>GGEPAWDSPLRRVLAELNRIPSSRRRAARLFEWLIAPMPPDHFYRRLWEREAVLVRRQDHTYYQGLFSTADLDSMLRNEEVQFGQHLDAARYINGRRETLNPPGRALPAAAWSLYQAGCSLRLLCPQAFSTTVWQFLAVLQEQFGSMAGSNVYLTPPNSQGFAPHYDDIEAFVLQLEGRKLWRVYRPRVPTEELALTSSPNFSQDDLGEPVLQTVLEPGDLLYFPRGFIHQAECQDGVHSLHLTLSTYQRNTWGDFLEAILPLAVQAAMEENVEFRRGLPRDFMDYMGAQHSDSKDPRRTAFMEKVRVLVARLGHFAPVDAVADQRAKDFIHDSLPPV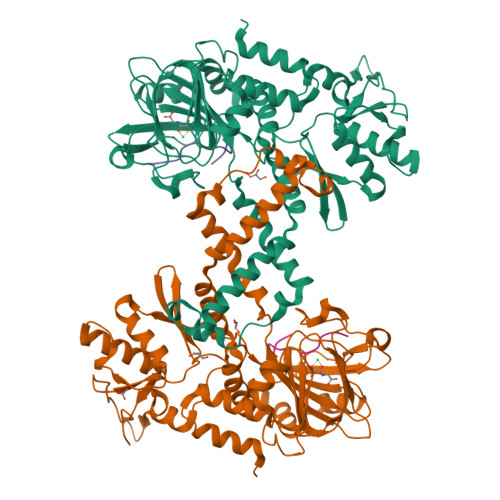LTDRERALSVYGLPIRWEAGEPVNVGAQLTTETEVHMLQDGIARLVGEGGHLFLYYTVENSRVYHLEEPKCLEIYPQQADAMELLLGSYPEFVRVGDLPCDSVEDQLSLATTLYDKGLLLTKMPLALN[2x];>[2x]GGGNHQHIGKP>[4x]MLTEFDAGYGEQPFRDLCANYPGAEAYDPHDFRIEWGPIFHRGRLDGSARVLIVGQDPAQHETIVRRILVGTAGRRTQGFLAKLGIVQSYVMVNTFLYSVYGQSGGSKHKNEPGIVDYRNKWFKAVLGPGNIEAVVSLGGLADEAWKAWLKSSDGAAYKTLAYQHITHPTWPESSAHDSATQAANTKIMLAKWNAALAALAPEVKHPDVPTTLVPYGDAFKPSE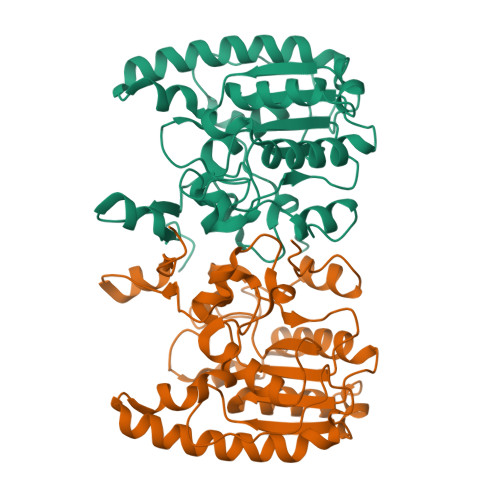LVDIIAKDLPAGLPAWMRGDTPWAVRQGVDAAAKRRTIMITIPDGVIP>MKLSDIYLELKKGYADSLLYSDLSLLVNIMEYEKDIDVMSIQSLVAGYEKSDTPTITCGIIVYNESKRIKKCLNSVKDDFNEIIVLDSYSTDDTVDIIKCDFPDVEIKYEKWKNDFSYARNKIIEYATSEWIYFIDADNLYSKENKGKIAKVARVLEFFSIDCVVSPYIEEYTGHLYSDTRRMFRLNGKVKFHGKVHEEPMNYNHSLPFNFIVNLKVYHNGYNPSE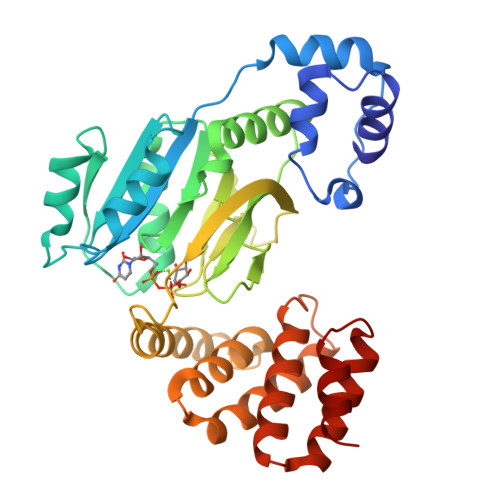NNIKSKTRRNINLTEEMLRLEPENPKWLFFFGRELHLLDKDEEAIDYLKKSINNYKKFNDQRHFIDALVLLCTLLLQRNNYVDLTLYLDILETEYPRCVDVDYFRSAIL[2x]>[5x]MGRAHKETLDKLTNAAINSINLLNTSKVKYLVSSAFAGLYVGIGILLIFTIGGLLTDAGSPMTKIVMGLSFAIALSLVIMTGTELFTGNNMVMSAGMLNKGVSIKDTSKIWAYSWVGNLIGALVLGIIFVGTGLVDKGPVAEFFANTAASKASMPFTALFF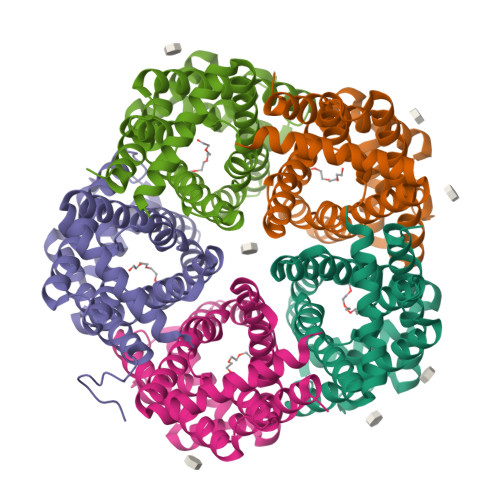RGILCNILVCVSVLCSFRTNSDTAKIIMIFLCLFAFITSGFEHSVANMTIYSVSLFSPTISTVTIGGAIYNLVAVTLGNIVGGALFMGLGTYILGKEKLNAAAENLY>MVLYFIGLGLYDERDITVKGLEIAKKCDYVFAEFYTSLMAGTTLGRIQKLIGKEIRVLSREDVELNFENIVLPLAKENDVAFMTPGDPLVATTHAELRIRAKRAGVESYVIHAPSIYSAVGI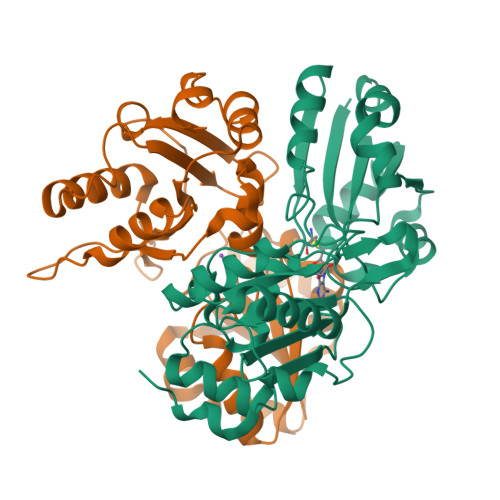TGLHIYKFGKSATVAYPEGNWFPTSYYDVIKENAERGLHTLLFLDIKAEKRMYMTANEAMELLLKVEDMKKGGVFTDDTLVVVLARAGSLNPTIRAGYVKDLIREDFGDPPHILIVPGKLHIVEAEYLVEIAGAPREILRVNV[2x]>MKVIEFHVVGNSLNQKPNKKILMWLVGLQNVFSHQLPRMPKEYITRLVFDPKHKTLALIKDGRVIGGICFRMFPSQGFTE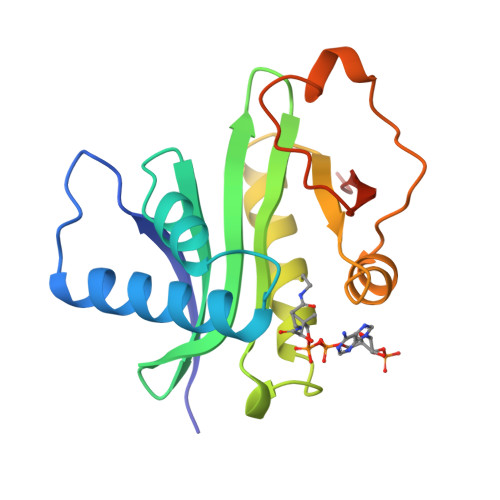IVFCAVTSNEQVKGYGTHLMNHLKEYHIKHDILNFLTYADEYAIGYFKKQGFSKEIKIPKTKYVGYIKDYEGATLMGCELNPRIPYTE[2x]>AEQSGISQTVIVGPWGAKVSTSSNGKAFDDGAFTGIREINLSYNKETAIGDLQVVYDLNGSPYVGQNHKSFITGFTPVKISLDFPSEYIMEVSGYTGNVSGYVVVRSLTFKTNKKTYGPYGVTSGTPFN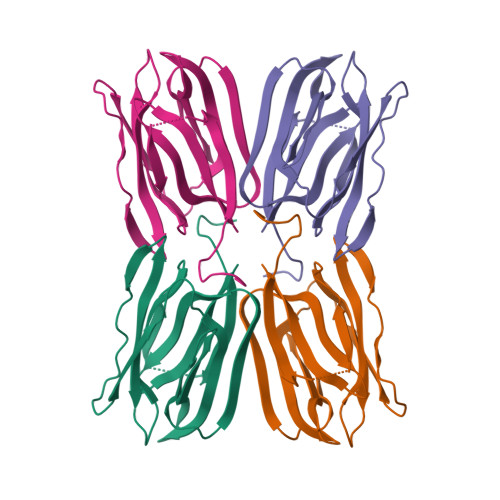LPIENGLIVGFKGSIGYWLDCFSMYLSL[2x]ARS2 is a direct interaction partner of CBC and together they form a platform for the assembly of co-transcriptional complexes that determine the fate of diverse RNA Pol II transcripts. Our structural analysis shows that ARS2 is made up of two regions, residues 147–270 and 408–763 that co-fold into a structured core with an intervening glutamate-rich region of unknown function that is likely unstructured. The human ARS2 core has an unusual structure comprising a largely helical ‘body’ from which project N- and C-terminal ‘legs’. We find that the RRM domain is required to bind RNA, whereas a basic patch in the C-terminal leg of ARS2 mediates the interaction with FLASH.

Here, we describe the crystal structure of the folded core of human ARS2 corresponding to residues 147–270 and 408–763, which are separated by a large unstructured region. We set out to determine the crystal structure of human ARS2 and first worked with the construct ARS2147–763, thus excluding the N- and C-terminal tails predicted to be unstructured. Since crystals of ARS2147–763 only diffracted to around 20 Å resolution, and disorder predictions suggested the presence of an additional central, low-complexity region, limited proteolysis was used to delineate the structured domains. Better crystals (space group P3121), diffracting to 3.7 Å resolution, were obtained by co-expression of two defined fragments denoted as ARS2147–270+408–763 in E. coli. The structure of ARS2147–270+408–763 was solved using selenomethionine-labelled protein and the single-isomorphous replacement with anomalous-scattering (SIRAS) method. The crystallised core, ARS2147–270+408–763, which lacks the central disordered region, retained identical ssRNA binding, whereas for ARS2147–270+494–763, missing the RRM domain as well, no significant RNA binding was detected with concentrations up to 50 µM ARS2 protein. In all crystal structures of hARS2 (except that with loop B deleted), only the first part of the loop is observed with 570-AEEEELL forming helix α10 (‘EEEE helix’). Remarkably, all crystal forms containing loop B, irrespective of space-group, exhibit the same intermolecular crystal contact, in which the acidic ‘EEEE helix’ and the preceding short β-strand pack into the positively charged cradle formed by the RRM β-sheet and the C-terminal extension of the RRM. To accommodate the same intermolecular contact in different crystal-packing environments, some angular flexibility of the loop B structure is required. Crystals of ARS2147–270+408–763Δ568–598 (Δloop B) diffracted to 3.37 Å resolution (space group C2221) and exhibited an ordered loop A. A composite model, including both loop A (from the ARS2147–270+408–763Δ568–598 structure) and most of loop B (from the ARS2147–270+408–763 structure) was artificially constructed and used for illustrative purposes since it is almost complete, only lacking residues 578–598.

>PVMKTFKEFLLSLDDSVDETEAVKRYNDYKLDFRRQQMQDFFLAHKDEEWFRSKYHPDEVGKRRQEARGALQNRLRVFLSLMETGWFDNLLLDIDKADAIVKMLDAAVIKMEGGTENDLRILEQ[2x];>[2x]GLECKPRPLHKTCSLFMRNIAPNISRAEIISLCKRYPGFMRVALSEPQPERRFFRRGWVTFDRSVNIKEICWNLQNIRLRECELSPGVNRDLTRRVRNINGITQHKQIVRNDIKLAAKLIHTLDDRTQLWASEPGTPPLPTSLPSQNPILKNITDYLIEEVSAEEEELLGSSGGAPPEEPPKEGNPAEINVERDEKLIKVLDKLLLYLRIVHSLDYYNTCEYPNEDEMPNRCGIIHVRGPMPPNRISHGEVLEWQKTFEEKLTPLLSVRESLSEEEAQKMGRKDPEQEVEKFVTSNTQELGKDKWLCPLSGKKFKGPEFVRKHIFNKHAEKIEEVKKEVAFFNNFLTDAKRPALPE>MSVEGLGKDFCGAIIPDNFFPIEKLRNYTQMGLIRDFAKGSAVIMPGEEITSMIFLVEGKIKLDIIFEDGSEKLLYYAGGNSLIGKLYPTGNNIYATAMEPTRTCWFSEKSLRTVFRTDEDMIFEIFKNYLTKVAYYARQVAEMNTYNPTIRILRLFYELCSSQGKRVGDTYEITMPLSQKSIGEITGVHHVTVSRVLACLKRENILDKKKNKIIVYNLGELKHLSEQTSYYSDPNSSSVDKLAAALDHH[6x]

The transcriptional regulator CprK from Desulfitobacterium spp. induces expression of halorespiratory genes upon binding of o-chlorophenol ligands and is reversibly inactivated by oxygen through disulphide bond formation. The CprK associated with the o-chlorophenolacetic acid (OCPA) reductive dehalogenase (CprAB) from D. dehalogenans and the closely related D. hafniense has been shown to bind OCPA with μM affinity leading to sequence-specific DNA-binding, and ultimately transcriptional activation of the associated cpr gene cluster (Pop et al., 2004; 2006; Gabor et al., 2006; Joyce et al., 2006; Mazon et al., 2007). Members of this family are homodimeric and contain an N-terminal sensor domain linked via a long α-helix (involved in formation of the dimer interface) to the C-terminal helix–turn–helix (HTH) DNA-binding domain. We here present crystal structures of the oxidized ligand-free (3.2 Å) and reduced ligand-free (2.0 Å), OCPA-bound (1.8 Å) and DNA-bound (1.8 Å) D. hafniense CprK in addition to an intermediate OCPA-bound structure obtained by soaking ligand-free crystals (2.0 Å).

Crystals of the oxidized, ligand-free wild-type CprK were difficult to obtain and only yielded data to low resolution (to 3.2 Å) using microfocus beamlines. Nevertheless, the relative position of the individual domains could be unambiguously determined and is roughly identical for the three individual dimers present in the asymmetric unit. It thus appears that considerable flexibility in the DNA-binding domain positions, and presumably in the entire molecule as a consequence, is lost upon oxidization, confirming the previously observed effect of limited proteolysis as detected by mass spectrometry. In case of CprK, oxidation leads to severe constraints on the position of the DNA-binding domains and hence a reduction in overall flexibility. Furthermore, while it does appear to not significantly affect ligand binding mode (13–14 and this work), it prohibits formation of the appropriate inter-domain contact network that establishes the DNA-binding form, thus inactivating transcription under aerobic conditions. However, the Cys-11 and Cys-200 residues of opposite monomers, respectively, part of each of these mobile structural elements, are likely to be in close proximity for most of the time. This explains the marked susceptibility of CprK for inactivation by oxygen through formation of the intermolecular Cys-11–Cys-200 disulphide bridges. Inactivation of CprK under aerobic conditions through Cys-11–Cys-200 disulphide bond formation is readily observed in vitro, although it remains unclear whether this process has physiological relevance.>[2x]QAQITGRPEWIWLALGTALMGLGTLYFLVKGMGVSDPDAKKFYAITTLVPAIAFTMYLSMLLGYGLTMVPFGGEQNPIYWARYADWLFTTALLLLDLALLVDADQGTILALVGAD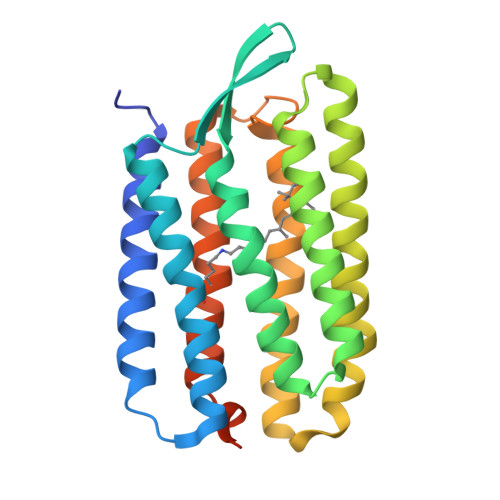GIMIGTGLVGALTKVYSYRFVWWAISTAAMLYILYVLFFGFTSKAESMRPEVASTFKVLRNVTVVLWSAYPVVWLIGSEGAGIVPLNIETLLFMVLDVSAKVGFGLILLRSRAIFGEAEAPEPSAGDGAAATSD>SNAMSQQFDLVVIGGGPGGYEAAIRAAQLGFKVACIEKRIHNGKPSLGGTCLNVGCIPSKALLDSSHRYEDTVHHLADHGITTGEVNFDLAKLLARKDKIVDQLTGGIDQLLKGNGIEWLKGTGKLLAGKKVEFVPHEGETQILEPKYVILASGSVPVNIPVAPVDQDIIVDSTGALNFPEVPKRLGVIGAGVIGLELGSVWRRLGAEVVVFEAMDAFLPMADKALSKEYQKILTKQGLDIRIGAKVSGTEVNGREVTVKYTQAGEDKEQ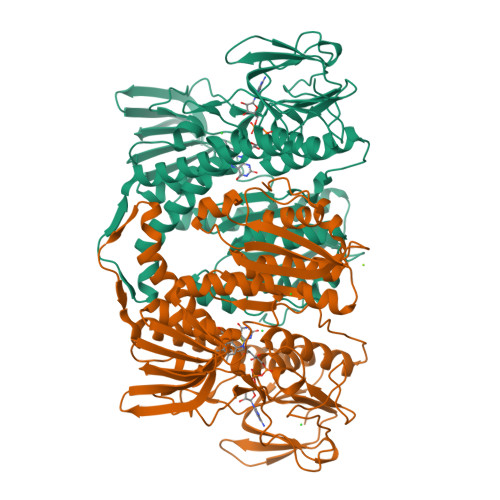TFDKLIVCVGRKAYAEGLLAEDSGIKLTERGLVEVNDHCATSVEGVYAIGDLVRGPMLAHKAMEEGVMAVERIHGHAAQVNYDTIISIIYTHPEAAWVGLTEEQAKEKGHEVKTGQFGFAVNGRALAAGEGAGFVKFVADAKTDRLLGMHVIGPAASDIVHQGMIALEFVSSVEDLQLMTFGHPTFSEVVHEAALAVDGRAIHAIQRKRK[4x]> GLGPLQIWQTDFTLEPRMAPRSWLAVTVDTASSAIVVTQHGRVTSVAAQHHWATA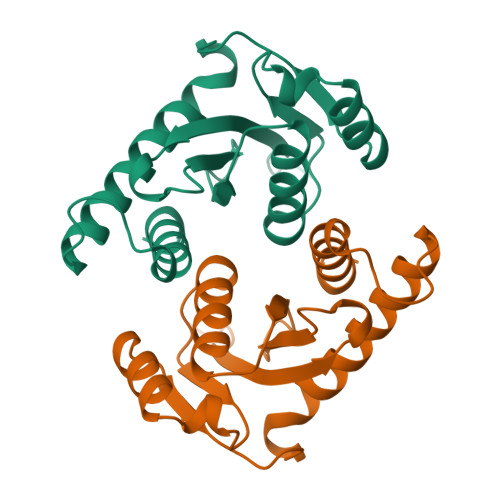IAVLGRPKAIKTDNGSCFTSKSTREWLARWGIAHTTGIPGNSQGQAMVERANRLLKDKIRVLAEGDGFMKRIPTSKQGELLAKAMYALNHF>MKEGKHFVLVHGACHGGWSWYKLKPLLEAAGHKVTALDLAASGTDLRKIEELRTLYDYTLPLMELMESLSADEKVILVGHSLGGMNLGLAMEKYPQKIYAAVFLAAFMPDSVHNSSFVLEQYNERTPAENWLDTQFLPYGSPEEPLTSMFFGPKFLAHKLYQLCSPEDLALASSLVRPSSLFMEDLSKAKYFTDERFGSVKRVYIVCTE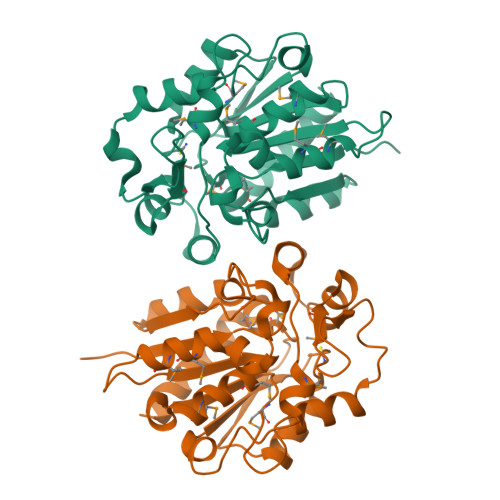DKGIPEEFQRWQIDNIGVTEAIEIKGADHMAMLCEPQKLCASLLEIAHKYNLEHHHHHH[8x]N-benzyl-1-{2-chloro-5-[(2-chloro-5-{5-(methylsulfonyl)-1-[3-(morpholin-4-yl)propyl]-4,5,6,7-tetrahydro-1H-pyrazolo[4,3-c]pyridin-3-yl}phenyl)ethynyl]phenyl}methanamine 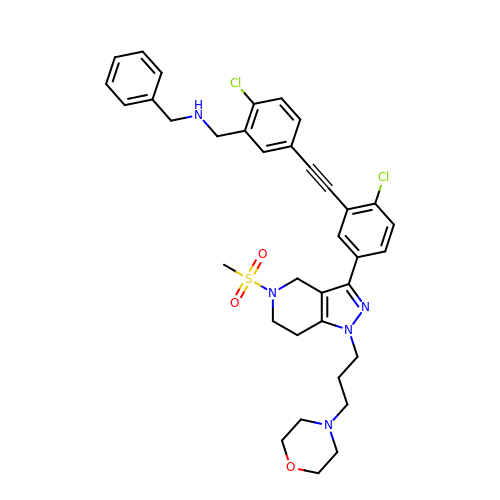| C36 H39 Cl2 N5 O3 S | IZBBHSKSQLPYHT-UHFFFAOYSA-N>[4x]MRGSHHHHHHGSAEPPNMPSMAPVLKNIMPAIVNVAVQGYLPNDVTPPGSAGNDEENQPNNRPPQSRMPEKGRKFESIGSGVIIDPNNGVIITNDHVIRNASLITVTLQDGRRLKA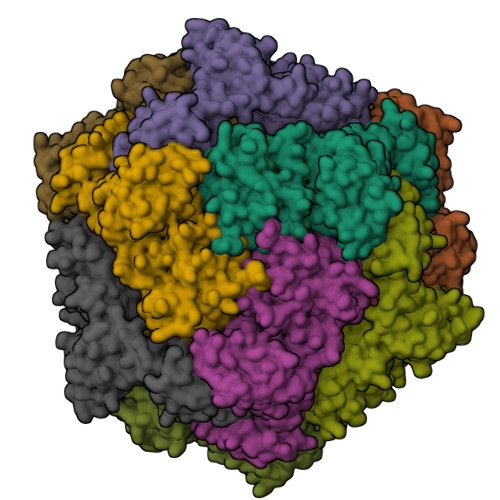RLIGGDSETDLAVLKIDAKNLKSLVIGDSDKLEVGDFVVAIGNPFGLNSFGNSQSATFGIVSALKRSDLNIEGVENFIQTDAAIGGGNSGGALVNAKGELIGINTAILSPYGGNVGIGFAIPINMVKDVAQQIIKFGSIHRGLMGIFVQHLTPELAQAMGYPEDFQGALVSQVNPNSPAELAGLKAGDIITQINDTKITQATQVKTTISLLRVGSTVKIIVERDNKPLTLSAVVTDIKSHEQKLQSNNPFLYGLALRAFEQESPPHGNVIGVQVVGASENSAGWRAGIRPGDIIISANKKPVTDVKSLQTIAQEKKKELLVQVLRGPGSMYLLVI>GDWHCDTKWMGDHVITKSTRTWVLPTYGNHLYGPINFDGTTGSGANAAYAGYKTPWGYFDFNRFHCHFSPRDWQRLINNHTGIRPKGLKIKVFNVQVKEVTTQDSTKTIANNLTSTVQIFADENYDLPYVLGSAT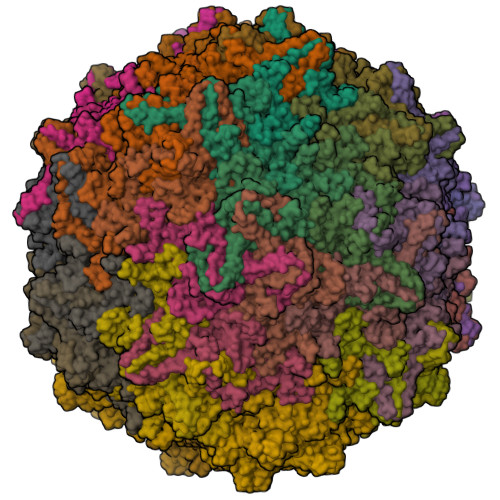QGTFPPFPNDVFMLPQYAYCTLQGNSGKFVDRSAFYCLEYFPSQMLRTGNNFEFQFKFEEVPFHSGWAQSQSLDRLMNPLLDQYLIGDYGTDASGNLIYHRAGPNDLNEFYKNWAPAPYECIQNINSSDNTKNANSINGSNSTNKWGLQGRQAWDAPGFVQASTYEGAAAGQSLLNGVLTFDKSSATTSSPAATAVNRTIEDEIQGTNNFGNARNNIVAINQQTKGTNPTTGSTSQFETMPGMVWSNRDIYLQGPIWAKIPNTDGHFHPSPRMGGFGLKHPPPMILIKNTPVPADPPTTFNPMPQTSFITEYSTGQVTVEMLWEVQKESSKRWNPEVQFTSNFGTSDPAVDGIPFGINNLGTYVESRPIGTRYISKHL[60x]>[22x]MYTNSDFVVIKALEDGVNVIGLTRGADTRFHHSEKLDKGEV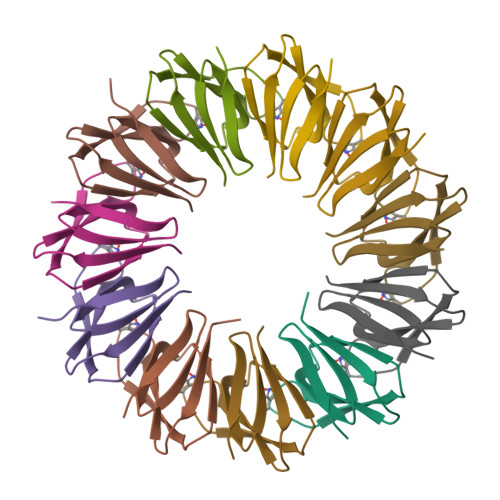LIAQFTEHTSAIKVRGKAYIQTRHGVIESEGKK> DMFLYNLTLQRATGISFAIHGNFSGTKQQEIVVSRGKILELLRPDPNTGKVHTLLTVEVFGVIRSLMAFRLTGGTKDYIVVGSDSGRIVILEYQPSKNMFEKIHQETFGKSGCRRIVPGQFLAVDPKGRAVMISAIEKQKLVYILNRDAAARLTISSPLEAHKANTLVYHVVGVDVGFENPMFACLEMDYEEADNDPTGEAAANTQQTLTFYELDLGLNHVVRKYSEPLEEHGNFLITVPGGSDGPSGVLICSENYITYKNFGDQPDIRCPIPRRRNDLDDPERGMIFVCSATHKTKSMFFFLAQTEQGDIFKITLETDEDMVTEIRLKYFDTVPVAAAMCVLKTGFLFVASEFGNHYLYQIAHLGDDDEEPEFSSAMPLEEGDTFFFQPRPLKNLVLVDELDSLSPILFCQIADLANEDTPQLYVACGRGPRSSLRVLRHGLEVSEMAVSELPGNPNAVWTVRRHIEDEFDAYIIVSFVNATLVLSIGETVEEVTDSGFLGTTPTLSCSLLGDDALVQVYPDGIRHIRADKRVNEWKTPGKKTIVKCAVNQRQVVIALTGGELVYFEMDPSGQLNEYTERKEMSADVVCMSLANVPPGEQRSRFLAVGLVDNTVRIISLDPSDCLQPLSMQALPAQPESLCIVEMGGTEKQDELGERGSIGFLYLNIGLQNGVLLRTVLDPVTGDLSDTRTRYLGSRPVKLFRVRMQGQEAVLAMSSRSWLSYSYQSRFHLTPLSYETLEFASGFASEQCPEGIVAISTNTLRILALEKLGAVFNQVAFPLQYTPRKFVIHPESNNLIIIETDHNAYTEATKAQRKQQMAEEMVEAAGEDERELAAEMAAAFLNENLPESIFGAPKAGNGQWASVIRVMNPIQGNTLDLVQLEQNEAAFSVAVCRFSNTGEDWYVLVGVAKDLILNPRSVAGGFVYTYKLVNNGEKLEFLHKTPVEEVPAAIAPFQGRVLIGVGKLLRVYDLGKKKLLRKCENKHIANYISGIQTIGHRVIVSDVQESFIWVRYKRNENQLIIFADDTYPRWVTTASLLDYDTVAGADKFGNICVVRLPPNTNDEVDEDPTGNKALWDRGLLNGASQKAEVIMNYHVGETVLSLQKTTLIPGGSESLVYTTLSGGIGILVPFTSHEDHDFFQHVEMHLRSEHPPLCGRDHLSFRSYYFPVKNVIDGDLCEQFNSMEPNKQKNVSEELDRTPPEVSKKLEDIRTRYAFDYKDD;> MTDRYTIHSQLEHLQSKYIGTGHADTTKWEWLVNQHRDSYCSYMGHFDLLNYFAIAENESKARVRFNLMEKMLQPCGPPADKPEEN;> MAKIAKTHEDIEAQIREIQGKKAALDEAQGVGLDSTGYYDQEIYGGSDSRFAGYVTSIAATELEDDDDDYSSSTSLLGQKKPGYHAPVALLNDIPQSTEQYDPFAEHRPPKIADREDEYKKHRRTMIISPERLDPFADGGKTPDPKMNARTYMDVMREQHLTKEEREIRQQLAEKAKAGELKVVNGAAASQPPSKRKRRWDQTADQTPGATPKKLSSWDQAETPGHTPSLRWDETPGRAKGSETPGATPGSKIWDPTPSHTPAGAATPGRGDTPGHATPGHGGATSSARKNRWDETPKTERDTPGHGSGWAETPRTDRGGDSIGETPTPGASKRKSRWDETPASQMGGSTPVLTPGKTPIGTPAMNMATPTPGHIMSMTPEQLQAWRWEREIDERNRPLSDEELDAMFPEGYKVLPPPAGYVPIRTPARKLTATPTPLGGMTGFHMQTEDRTMKSVNDQPSGNLPFLKPDDIQYFDKLLVDVDESTLSPEEQKERKIMKLLLKIKNGTPPMRKAALRQITDKAREFGAGPLFNQILPLLMSPTLEDQERHLLVKVIDRILYKLDDLVRPYVHKILVVIEPLLIDEDYYARVEGREIISNLAKAAGLATMISTMRPDIDNMDEYVRNTTARAFAVVASALGIPSLLPFLKAVCKSKKSWQARHTGIKIVQQIAILMGCAILPHLRSLVEIIEHGLVDEQQKVRTISALAIAALAEAATPYGIESFDSVLKPLWKGIRQHRGKGLAAFLKAIGYLIPLMDAEYANYYTREVMLILIREFQSPDEEMKKIVLKVVKQCCGTDGVEANYIKTEILPPFFKHFWQHRMALDRRNYRQLVDTTVELANKVGAAEIISRIVDDLKDEAEQYRKMVMETIEKIMGNLGAADIDHKLEEQLIDGILYAFQEQTTEDSVMLNGFGTVVNALGKRVKPYLPQICGTVLWRLNNKSAKVRQQAADLISRTAVVMKTCQEEKLMGHLGVVLYEYLGEEYPEVLGSILGALKAIVNVIGMHKMTPPIKDLLPRLTPILKNRHEKVQENCIDLVGRIADRGAEYVSAREWMRICFELLELLKAHKKAIRRATVNTFGYIAKAIGPHDVLATLLNNLKVQERQNRVCTTVAIAIVA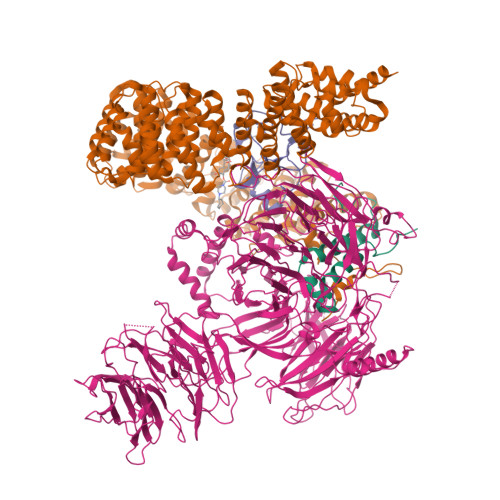ETCSPFTVLPALMNEYRVPELNVQNGVLKSLSFLFEYIGEMGKDYIYAVTPLLEDALMDRDLVHRQTASAVVQHMSLGVYGFGCEDSLNHLLNYVWPNVFETSPHVIQAVMGALEGLRVAIGPCRMLQYCLQGLFHPARKVRDVYWKIYNSIYIGSQDALIAHYPRIYNDDKNTYIRYELDYIL;> DLIFCRKQAGVAIGRLCEKCDGKCVICDSYVRPCTLVRICDECNYGSYQGRCVICGGPGVSDAYYCKECTIQEKDRDGCPKIVNL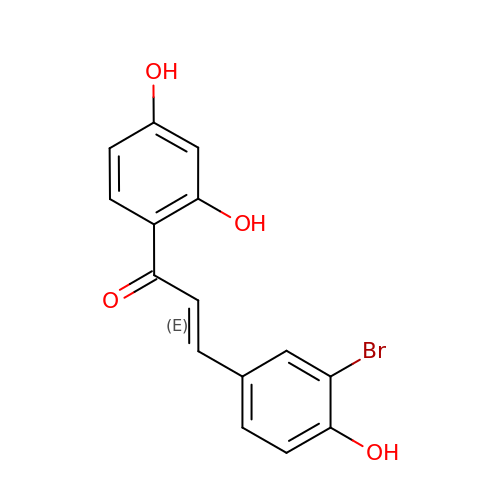(~{E})-1-[2,4-bis(oxidanyl)phenyl]-3-(3-bromanyl-4-oxidanyl-phenyl)prop-2-en-1-one | C15 H11 Br O4 | YOXIGWQDHRYVTE-ORCRQEGFSA-N>GSAMASNAVLYKSNHNVVYSCKYHIVWCPKYRRKVLVGAVEMRLKEIIQEVAKELRVEIIEMQTDKDHIHILADIDPSFGVMKFIKTA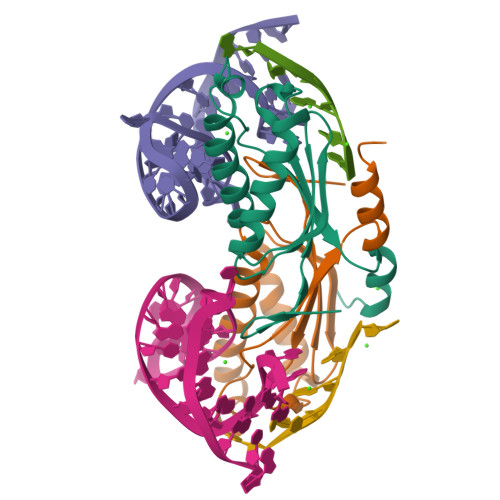KGRSSRILRQEFNHLKTKLPTLWTNSCFISTVGGAPLNVVKQYIENQQNSNRPKQKEKWKSYVDNLQTKAL[4x]> MKHHHHHHP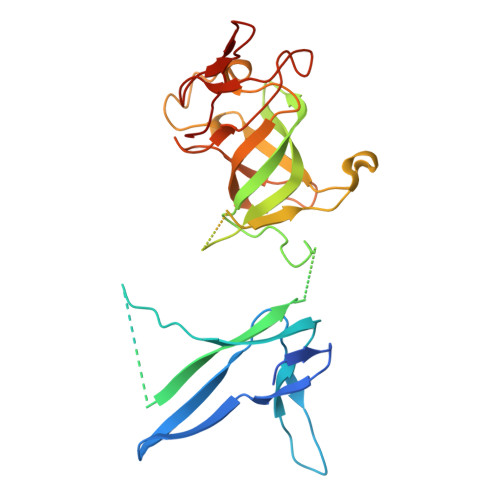MACNFQFPEIAYPGKLICPQYGTENKDGEDIIFNYVPGPGTKLIQYEHNGRTLEAITATLVGTVRCEEEKKTDQEEEREGTDQSTEEEKSVDASPNDVTRRTVKNILVSVLPGTEKGRKTNKYANNDFANNLPKEGDIVLTRVTRLSLQRANVEILAVEDKPSPIDSGIGSNGSGIVAAGGGSGAATFSVSQASSDLGETFRGIIRSQDVRSTDRDRVKVIECFKPGDIVRAQVLSLGDGTNYYLTTARNDLGVVFARAANGAGGLMYATDWQMMTSPVTGATEKRKCAKPF> QICPKRCVCQILSPNLATLCAKKGLLFVPPNIDRRTVELRLADNFVTNIKRKDFANMTSLVDLTLSRNTISFITPHAFADLRNLRALHLNSNRLTKITNDMFSGLSNLHHLILNNNQLTLISSTAFDDVFALEELDLSYNNLETIPWDAVEKMVSLHTLSLDHNMIDNIPKGTFSHLHKMTRLDV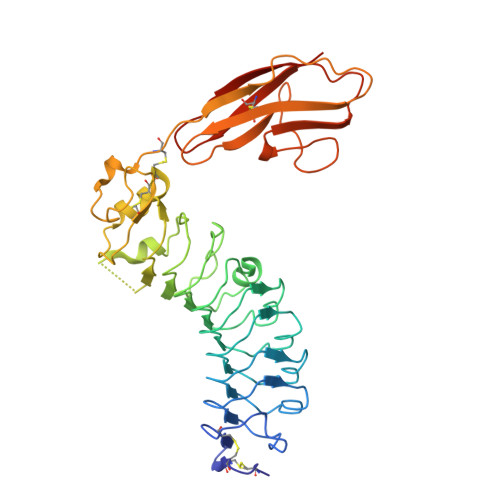TSNKLQKLPPDPLFQRAQVLATSGIISPSTFALSFGGNPLHCNCELLWLRRLSREDDLETCASPPLLTGRYFWSIPEEEFLCEPPLITRHTHEMRVLEGQRATLRCKARGDPEPAIHWISPEGKLISNATRSLVYDNGTLDILITTVKDTGAFTCIASNPAGEATQIVDLHIIKLPHHHHHH>[4x]MLDMPIDPVYYQLAEYFDSLPKFDQFSSAREYREAINRIYEERNRQLSQH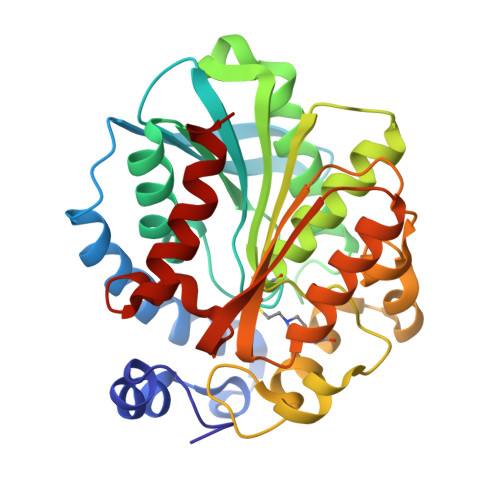ERVERVEDRTIKGRNGDIRVRVYQQKPDSPVLVYYHGGGFVICSIESHDALCRRIARLSNSTVVSVDYRLAPEHKFPAAVYDCYDATKWVAENAEELRIDPSKIFVGGDSAGGNLAAAVSIMARDSGEDFIKHQILIYPVVNFVAPTPSLLEFGEGLWILDQKIMSWFSEQYFSREEDKFNPLASVIFADLENLPPALIITAEYDPLRDEGEVFGQMLRRAGVEASIVRYRGVLHGFINYYPVLKAARDAINQIAALLVFD> MLRRAYIQRRYPFNKRGPREHKSWKHHVLTEPPKPLQWRDPKVWTRDLSVMKSFDAPQWDLWQSRPRSEDMDEALQPFMDMPKSLKDRRYDIPWWANPFGAWYLQNILSLELLKLKSKTNAEKIATYRSYMRSLASGKDNTMSDDDVIRNIIKERWKTLEFGDRNAGYPCTFGDYIQFLNEWFKSLDEEGMQRLREHFDRRIRPLLAVMSPVDILWLEALTQNSPHNKEQLQRKIAFQTSLGTPEFFDMSKRLRYEINEDYKVRDELGPELFALWSKAPERWPPERLSKMYGLDFTLVRKILVWHHF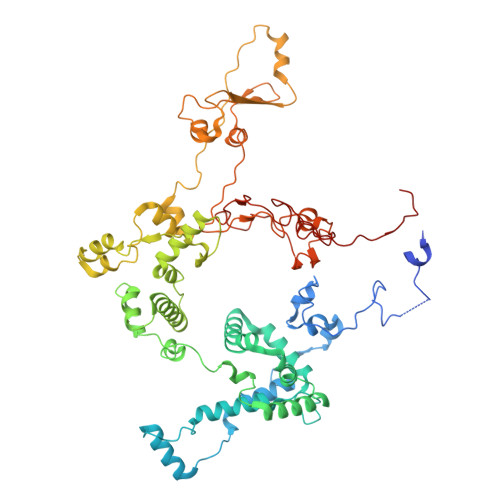KACYDACVEPDWSLPKRLFALEWIRDVRARKHGLFYGKMRFAEQKITFYSDRFLFRDLVNRREASYANVWEMDDPYRFLQTEQDYEDYWGDNYDVYRRMFPEMIGRTGEPVQQYGQMPIWAGPHRQHANKSEHNWMFAEIGVNVGHEALKKLELDPTNEKRRRFVIRQPDGTLRSAKMSEMRAWYWKEEWADFRFWAPQMEWGIENTPSQEQYQEHVPDTTDADFRKQRRIQSRPVKWFYESHYTRTGSFAGFQPLRFMQRRTEREVRWPDVINAAVQIQKRKPAAYIFKAIPEL> GPLGSEAHLYMQVQIVAEDQFCGHQGNDMYDEEKVKYTVFKVLKNSSLAEFVQSLSQTMGFPQDQIRLWPMQARSNGTKRPAMLDNEADGNKTMIELSDNENPWTIFLETVDPELAASGATLPKFDKDHDVMLFLKMYDPKTRSLNYCGHIYTPISCKIRDLLPVMCDRAGFIQDTSLILYEEVKPNLTERIQDYDVSLDKALDELMDGDIIVFQKDDPE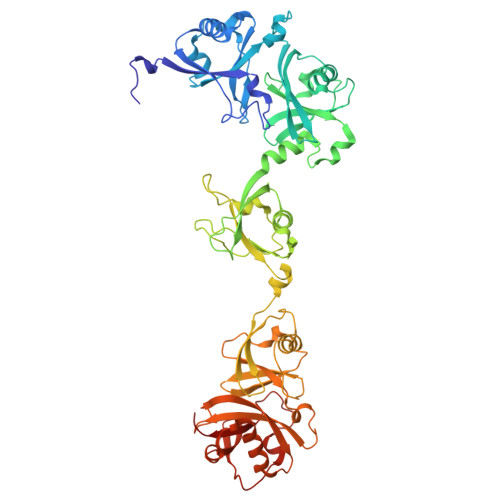NDNSELPTAKEYFRDLYHRVDVIFCDKTIPNDPGFVVTLSNRMNYFQVAKTVAQRLNTDPMLLQFFKSQGYRDGPGNPLRHNYEGTLRDLLQFFKPRQPKKLYYQQLKMKITDFENRRSFKCIWLNSQFREEEITLYPDKHGCVRDLLEECKKAVELGEKASGKLRLLEIVSYKIIGVHQEDELLECLSPATSRTFRIEEIPLDQVDIDKENEMLVTVAHFHKEVFGTFGIPFLLRIHQGEHFREVMKRIQSLLDIQEKEFEKFKFAIVMMGRHQYINEDEYEVNLKDFEPQPGNMSHPRPWLGLDHFNK> MGIALGMIETRGLVPAIEAADAMTKAAEVRLIGREFVGGG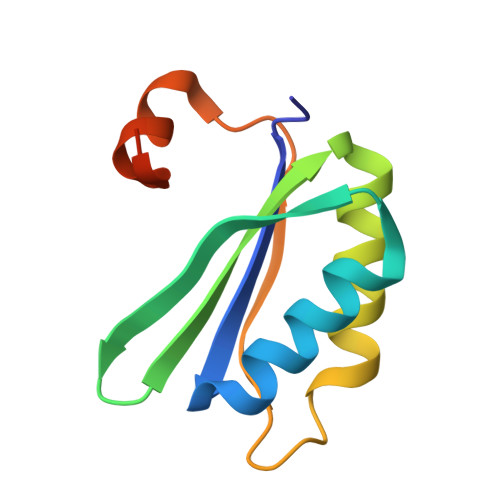YVTVLVRGETGAVNAAVRAGADACERVGDGLVAAHIIARPHREVEPALGNGDFLGQKD> GKTMKMRKFTIADASLERSPGQEADISVGNLVDERHGGPITIGYGRYAPGQSLTETMAVDDVMIVLEGRLSVSTDGETVTAGPGEIVYMPKGETVTIRSHEEGALTAYVTYPHWR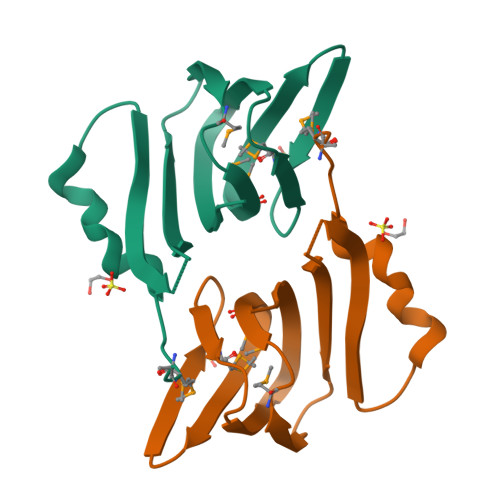PAHA> GAMGSDSNSDN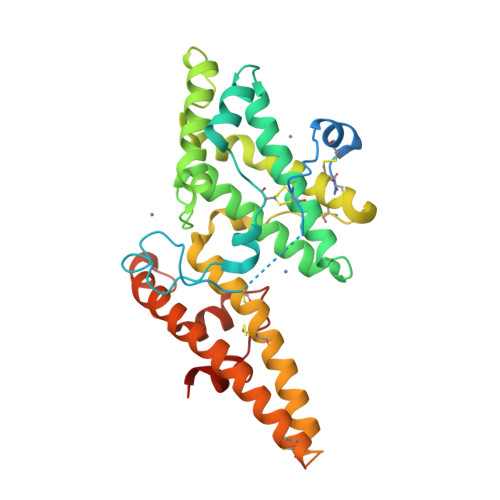SNQNIFPDGSELAGGIPRSIYTINLGFNKCPTEEICKDFSNLPQCRKNVHERNNWLGSSVKNFSSDNKGVLVPPRRQSLCLRITLQDFRTKKKKEGDFEKFIYSYASSEARKLRTIHNNNLEKAHQAIRYSFADIGNIIRGDDMMDTPTSKETITYLEKVLKIYNENNDKPKDAKKWWTENRHHVWEAMMCGYQSAQKDNQCTGYGNIDDIPQFLRWFREWGTYVCEESEKNMNTLKAVCFPKQPRTEANPALTVHENEMCSSTLKKYEEWYNKRKTEWTEQSIKYNNDKINYTDIKTLSPSEYLIEKCPECKCTKKNLQDVFELTFD>[2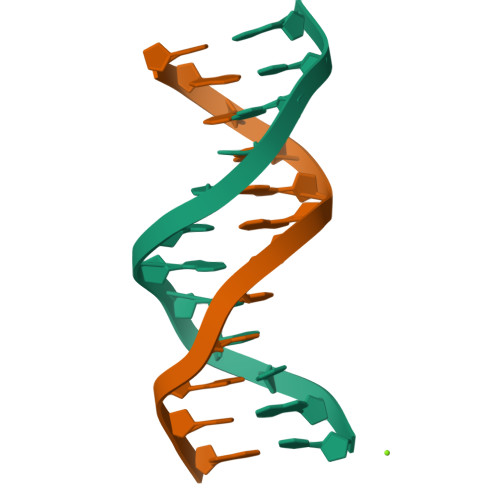x]CGTAGATCTACG N-(6-{[3-(4-BROMOPHENYL)-1,2-BENZISOTHIAZOL-6-YL]OXY}HEXYL)-N-METHYLPROP-2-EN-1-AMINE | C23 H27 Br N2 O S | 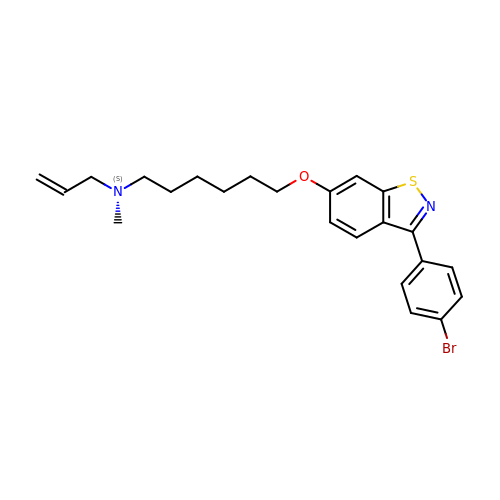UCIDPJLYUKNYFZ-UHFFFAOYSA-N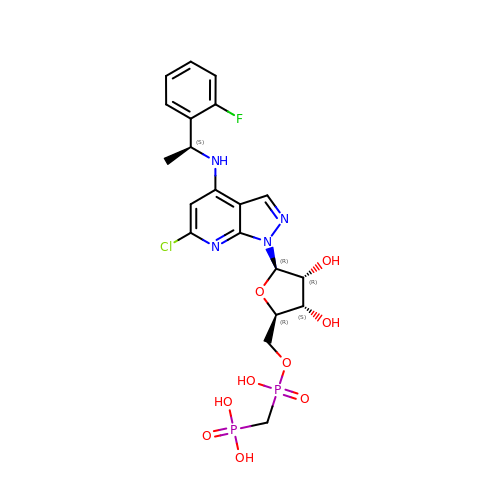[[(2~{R},3~{S},4~{R},5~{R})-5-[6-chloranyl-4-[[(1~{S})-1-(2-fluorophenyl)ethyl]amino]pyrazolo[3,4-b]pyridin-1-yl]-3,4-bis(oxidanyl)oxolan-2-yl]methoxy-oxidanyl-phosphoryl]methylphosphonic acid | C20 H24 Cl F N4 O9 P2 | MFYLCAMJNGIULC-KCVUFLITSA-N> KTNENVISFFDSTDAETQNHDVLMKGCGEFIVNLRTLLRTFRTITDNWILQANTKTPITDLTNTTD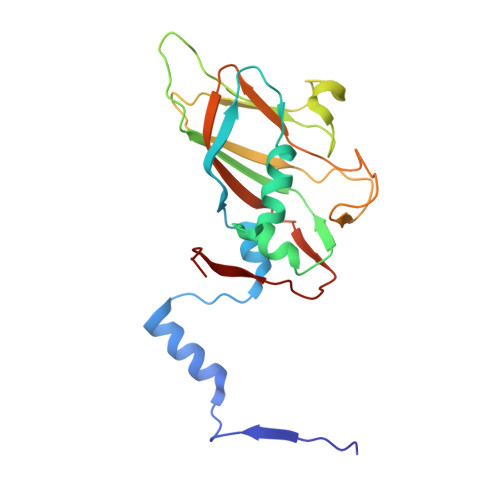AQGRDYMSYLSYLYRFYRGGRRYKFFNTTPLKQSQTCYIRSFLMPRNYSADEINVDGPSHITYPVINPVHEVEVPFYSQYRKIPIASTSDKGYDSSLMYFSNTSTTQIVARAGNDDFTFGWMIGPPQLQGETRSVVP>ETTDSFWEVGNYKRTVKRIDDGHRLCNDLMNCVQERAKIEKAYGQQLTDWAKRWRQLIEKGPQYGSLERAWGAIMTEADKVSELHQEVKNNLLNEDLEKVKNWQKDAYHKQIMGGFKETKEAEDGFRKAQKPWAKKMKELEAAKKAYHLACKEEKLAMTREMNSKTEQSVTPEQQKKLQDKVDKCKQDVQKTQ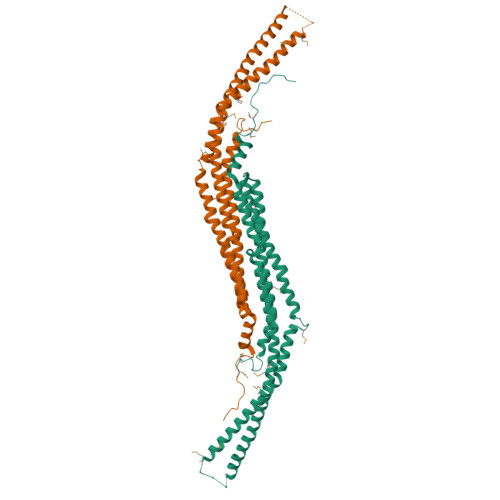EKYEKVLEDVGKTTPQYMENMEQVFEQCQQFEEKRLVFLKEVLLDIKRHLNLAENSSYIHVYRELEQAIRGADAQEDLRWFRSTSGPGMPMNWPQFEEWNPD[6x]N-{[4-(methanesulfonyl)phenyl]methyl}-N'-{[(3R)-oxolan-3-yl]methyl}urea | 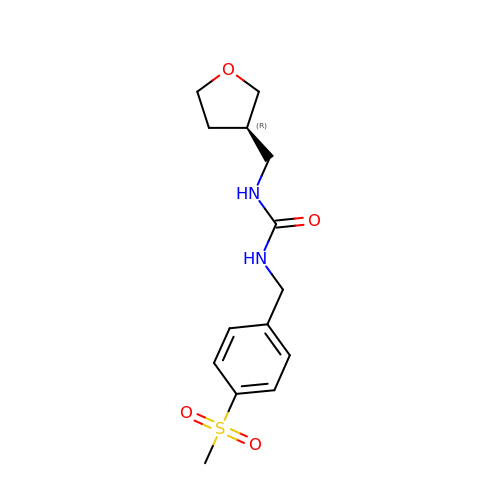C14 H20 N2 O4 S | KXBPKQJBIPGTRF-GFCCVEGCSA-N>[4x]MTWLPLNPIPLKDRVSMIFLQYGQIDVIDGAFVLIDKTGIRTHIPVGSVACIMLEPGTRVSHAAVRLAAQVGTLLVWVGEAGVRVYASGQPGGARSDKLLYQAKLALDEDLRLKVVRKMFELRFGEPAPARRSVEQLRGIEGSRVRATYALLAKQYGVTWNGRRYDPKDWEKGDTINQCISAATSCLYGVTEAAILAAGYA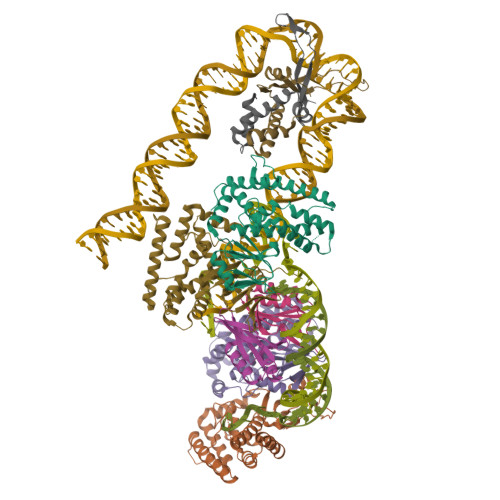PAIGFVHTGKPLSFVYDIADIIKFDTVVPKAFEIARRNPGEPDREVRLACRDIFRSSKTLAKLIPLIEDVLAAGEIQPPAPPEDAQPVAIPLPVSLGDAGHRSS;>MSMLVVVTENVPPRLRGRLAIWLLEVRAGVYVGDVSAKIREMIWEQIAGLAEEGNVVMAWATNTETGFEFQTFGLNRRTPVDLDGLRLVSFLPVGSSENLYFQ[2x];> MALTKAEMSEYLFDKLGLSKRDAKELVELFFEEIRRALENGEQVKLSGFGNFDLRDKNQRPGRNPKTGEDIPITARRVVTFRPGQKLKSRVENASPKDE;> MTKSELIERLATQQSHIPAKTVEDAVKEMLEHMASTLAQGERIEIRGFGSFSLHYRAPRTGRNPKTGDKVELEGKYVPHFKPGKELRDRANIYG>LRGFIIGRFQPFHKGHLEVIKKIAEEVDEII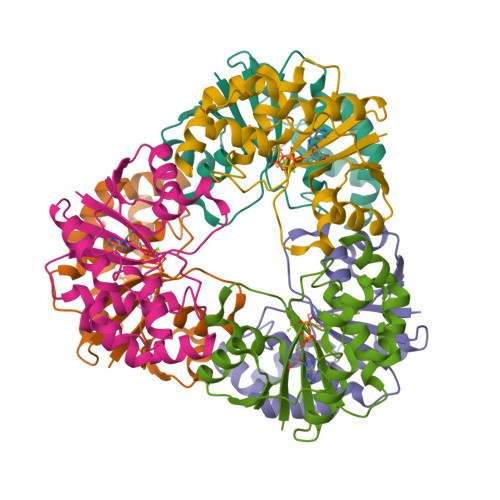IGIGSAQKSHTLENPFTAGERILMITQSLKDYDLTYYPIPIKDIEFNSIWVSYVESLTPPFDIVYSGNPLVRVLFEERGYEVKRPEMFNRKEYSGTEIRRRMLNGEKWEHLVPKAVVDVIKEIKGVERLRKLAQTDK[6x]> QETPAEIDPSKIPGEWRIIYAAADNKDKIVEGGPLRNYYRR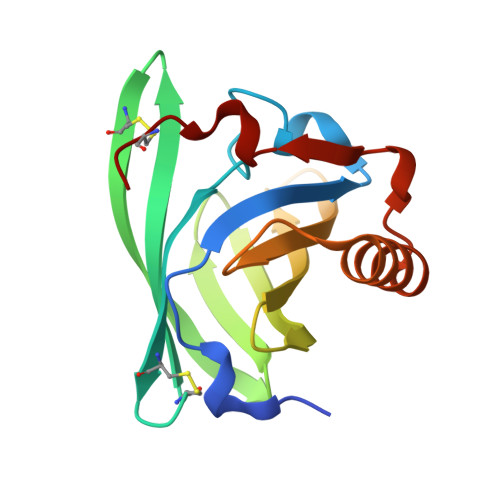IECINDCESLSITFYLKDQGTCLLLTEVAKRQEGYVYVLEFYGTNTLEVIHVSENMLVTYVENYDGERITKMTEGLAKGTSFTPEELEKYQQLNSERGVPNENIENLIKTDNCPP> MIVDFYFDFLSPFSYLANQRLSKLAQDYGLTIRYNAIDLARVKIAIGNVGPSNRDLKVKLDYLKVDLQRWAQLYGIPLVFPANYNSRRMNIGFYYSGAEAQAAAYVNVVFNAVWGEGIAPDLESLPALVSEKLGWDRSAFEHFLSSNAATERYDEQTHAAIERKVFG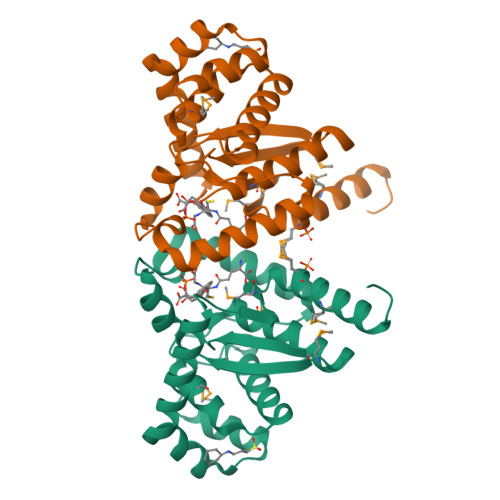VPTMFLGDEMWWGNDRLFMLESAMGRLCRQNADLSS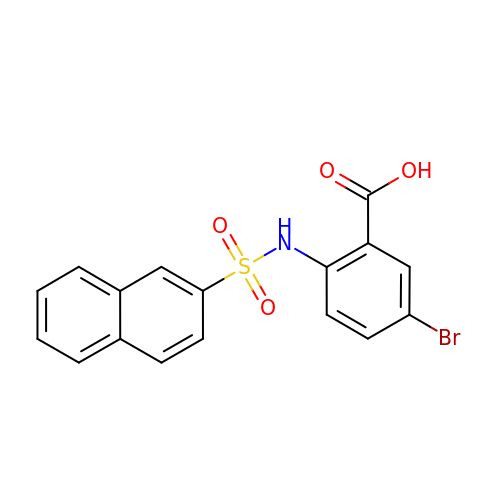5-bromanyl-2-(naphthalen-2-ylsulfonylamino)benzoic acid | C17 H12 Br N O4 S | PWDMGXXYINBNBW-UHFFFAOYSA-N> MAASGLDHLKNGYRRRFCRPSRARDINTEQGQNVLEILQDCFEEKSLANDFSTNSTKSVPNSTRKIKDTCIQSPSKECQKSHPKSVPVSSKKKEASLQFVVEPSEATNRSVQAHEVHQKILATDVSSKNTPDSKKISSRNINDHHSEADEEFYLSVGSPSVLLDAKTSVSQNVIPSSAQKRETYTFENSVNMLPSSTEVSVKTKKRLNFDDKVMLKKIEIDNKVSDEEDKTSEGQERKPSGSSQNRIRDSEYEIQRQAKKSFSTLFLETVKRKSESSPIVRHAATAPPHSCPPDDTKLIEDEFIIDESDQSFASRSWITIPRKAGSLKQRTISPAESTALLQGRKSREKHHNILPKTLANDKHSHKPHPVETSQPSDKTVLDTSYALIGETVNNYRSTKYEMYSKNAEKPSRSKRTIKQKQRRKFMAKPAEEQLDVGQSKDENIHTSHITQDEFQRNSDRNMEEHEEMGNDCVSKKQMPPVGSKKSSTRKDKEESKKKRFSSESKNKLVPEEVTSTVTKSRRISRRPSDWWVVKSEESPVYSNSSVRNELPMHHNSSRKSTKKTNQSSKNIRKKTIPLKRQKTATKGNQRVQKFLNAEGSGGIVGHDEISRCSLSEPLESDEADLAKKKNLDCSRSTRSSKNEDNIMTAQNVPLKPQTSGYTCNIPTESNLDSGEHKTSVLEESGPSRLNNNYLMSGKNDVDDEEVHGSSDDSKQSKVIPKNRIHHKLVLPSNTPNVRRTKRTRLKPLEYWRGERIDYQGRPSGGFVISGVLSPDTISSKRKAKENI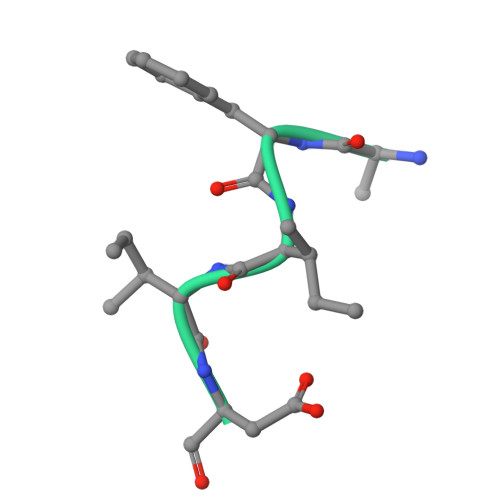GKVNKKSNKKRICLDNDERKTNLMVNLGIPLGDPLQPTRVKDPETREIILMDLVRPQDTYQFFVKHGELKVYKTLDTPFFSTGKLILGPQEEKGKQHVGQDILVFYVNFGDLLCTLHETPYILSTGDSFYVPSGNYYNIKNLRNEESVLLFTQIKR Protein arginine methyltransferases (PRMTs) are important therapeutic targets, playing a crucial role in the regulation of many cellular processes and being linked to many diseases. Then, another series of compounds (12a–12h) were designed and synthesized, introducing also an adenosine moiety and exploring the distance between the three groups. We also report crystal structures with various PRMTs supporting the observed specificity and selectivity. On the contrary, we were able to cocrystallize the compounds in the complex with both PRMT4 and PRMT6.

Structure determinations and refinements revealed that only compounds 12a, 12c, and 12f are visible in the active site of each monomer of the PRMT6 dimer. In all the structures of the complexes with PRMT6, the electron density for the compound is always better in one monomer. Compound 12a is the only one for which a complete electron density is visible in one monomer of the PRMT6 structure, whereas for 12c and 12f the electron density becomes fragmented after the guanidine group and the density for the methyl-4-hydroxy-2-naphthoate moiety is weak. Moreover, for compound 12f, the active site of one monomer is occupied by both the compound and SAH. The crystal structure revealed an unusual distorted U-shaped conformation adopted by compound 12a (and probably also 12c and 12f) in the binding to PRMT6, with a folding at the level of the guanidine group. Whereas the adenosine moiety lies into its canonic binding pocket, the guanidine group of the compounds is unable to reach the PRMT6 double-E loop clamp because the linker with the sugar is too short, even for the longer compound 12f. Instead of binding in the arginine substrate pocket as observed with PRMT4, the methyl-4 hydroxy-2-naphthoate moiety is sandwiched between the adenosine and the side chains of Y50 and Y51 residues of the α helix motif I. Hence, the binding of compounds 12a, 12c, and 12f affects the proper folding of the PRMT6 alpha-X helix containing the motif I (Y50-Y51-X-X-Y54).

>GHMAAPPRPRRTKSERDQLYYESYSDVSVHEEMIADQVRTEAYRLGILKNWAALRGKTVLDVGAGTGILSIFCAQAGARRVYAVEASAIWQQAREVVRLNGLEDRVHVLPGPVETVELPERVDAIVSEWMGYGLLHESMLSSVLHARTKWLKEGGLLLPASAELFVAPISDQMLEWRLGFWSQVKQHYGVDMSCMESFATRCLMGHSEIVVQDLSGEDVLARPQRFAQLELARAGLEQELEAGVGGRFRCSCYGSAPLHGFAVWFQVTFPGGDSEKPLVLSTSPLHPATHWKQALLYLNEPVPVEQDTDISGEITLLPSPDNPRRLRILLRYKVGDHEEKTKDFAMED[2x]> AAUUGAAGAGUUUGAUCAUGGCUCAGAUUGAACGCUGGCGGCAGGCCUAACACAUGCAAGUCGAACGGUAACAGGAAGAAGCUUGCUUCUUUGCUGACGAGUGGCGGACGGGUGAGUAAUGUCUGGGAAACUGCCUGAUGGAGGGGGAUAACUACUGGAAACGGUAGCUAAUACCGCAUAACGUCGCAAGACCAAAGAGGGGGACCUUCGGGCCUCUUGCCAUCGGAUGUGCCCAGAUGGGAUUAGCUAGUAGGUGGGGUAACGGCUCACCUAGGCGACGAUCCCUAGCUGGUCUGAGAGGAUGACCAGCCACACUGGAACUGAGACACGGUCCAGACUCCUACGGGAGGCAGCAGUGGGGAAUAUUGCACAAUGGGCGCAAGCCUGAUGCAGCCAUGCCGCGUGUAUGAAGAAGGCCUUCGGGUUGUAAAGUACUUUCAGCGGGGAGGAAGGGAGUAAAGUUAAUACCUUUGCUCAUUGACGUUACCCGCAGAAGAAGCACCGGCUAACUCCGUGCCAGCAGCCGCGGUAAUACGGAGGGUGCAAGCGUUAAUCGGAAUUACUGGGCGUAAAGCGCACGCAGGCGGUUUGUUAAGUCAGAUGUGAAAUCCCCGGGCUCAACCUGGGAACUGCAUCUGAUACUGGCAAGCUUGAGUCUCGUAGAGGGGGGUAGAAUUCCAGGUGUAGCGGUGAAAUGCGUAGAGAUCUGGAGGAAUACCGGUGGCGAAGGCGGCCCCCUGGACGAAGACUGACGCUCAGGUGCGAAAGCGUGGGGAGCAAACAGGAUUAGAUACCCUGGUAGUCCACGCCGUAAACGAUGUCGACUUGGAGGUUGUGCCCUUGAGGCGUGGCUUCCGGAGCUAACGCGUUAAGUCGACCGCCUGGGGAGUACGGCCGCAAGGUUAAAACUCAAAUGAAUUGACGGGGGCCCGCACAAGCGGUGGAGCAUGUGGUUUAAUUCGAUGCAACGCGAAGAACCUUACCUGGUCUUGACAUCCACGGAAGUUUUCAGAGAUGAGAAUGUGCCUUCGGGAACCGUGAGACAGGUGCUGCAUGGCUGUCGUCAGCUCGUGUUGUGAAAUGUUGGGUUAAGUCCCGCAACGAGCGCAACCCUUAUCCUUUGUUGCCAGCGGUCCGGCCGGGAACUCAAAGGAGACUGCCAGUGAUAAACUGGAGGAAG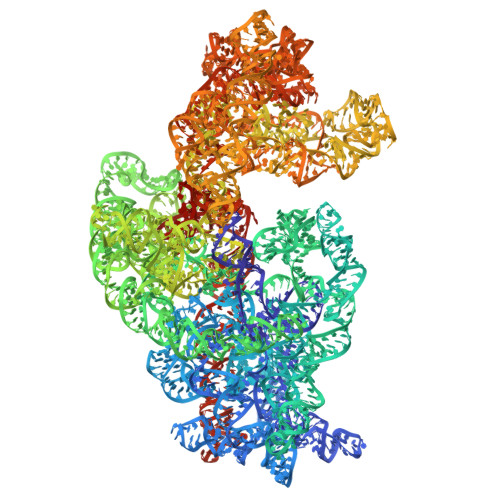GUGGGGAUGACGUCAAGUCAUCAUGGCCCUUACGACCAGGGCUACACACGUGCUACAAUGGCGCAUACAAAGAGAAGCGACCUCGCGAGAGCAAGCGGACCUCAUAAAGUGCGUCGUAGUCCGGAUUGGAGUCUGCAACUCGACUCCAUGAAGUCGGAAUCGCUAGUAAUCGUGGAUCAGAAUGCCACGGUGAAUACGUUCCCGGGCCUUGUACACACCGCCCGUCACACCAUGGGAGUGGGUUGCAAAAGAAGUAGGUAGCUUAACCUUCGGGAGGGCGCUUACCACUUUGUGAUUCAUGACUGGGGUGAAGUCGUAACAAGGUAACCGUAGGGGAACCUGCGGUUGGAUCA>DNSDNLRPVVIDGSNVAMSHGNKEEFSCRGIQLAVDWFLDKGHKDITVFVPAWRKEQSRPDAPITDQDILRKLEKEKILVFTPSRRVQGRRVVCYDDRFIVKLAFDSDGIIVSNDNYRDLQVEKPEWKKFIEERLLMYSFVNDKFMPPDDPLGR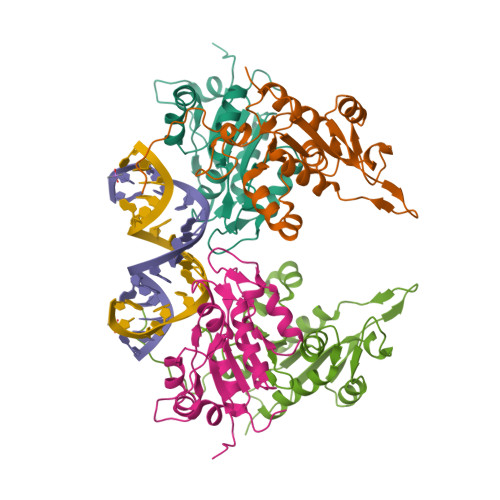HGPSLENFLRKRPIVPEHKKQPCP[2x]>MLKTNIELKPKVEAFLNEEIKMFINGEFVSAIGGKTFETYNPATEDVLAVVCEAQEEDIDAAVKAARSAFESGPWAEMTTAERAHLIYKLADLIEEHREELAQLEALDNGKPYQVALDDDISATVENYRYYAGWTTKIIGQTIPISKDYLNYTRHEPVGVVGQIIPWNFPLVMSSWKMGAALATGCTIVLKPASQTPLSLLYAAKLFKEAGFPNGVVNFVPGFGPEAGAAIVNHHDIDKVAFTGSTVTGKYIMRQSAEMIKHVTLELGGKSPNIILEDADLEEAINGAFQGIMYNHGQNCSAGSRVFVHRKHYETVVDALVKMANNVKLGAGMEKETEMGPLVSKKQQERVLNYIEQGKKEGATVA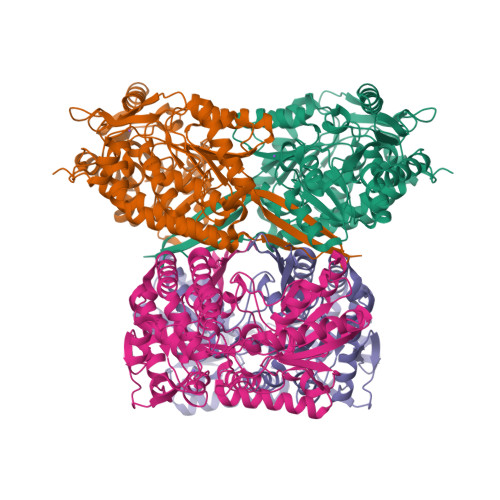AGGERALEKGYFVKPTVFTDVTDDMTIVKEEIFGPVVVVLPFDSTEEVIERANNSSYGLAAGVWTQNIKTGHQVANKLKAGTVWINDYNLENAAAPFGGYKQSGIGRELGSYALDNYTEVKSVWVNIK[12x]> PISPIETVPVKLKPG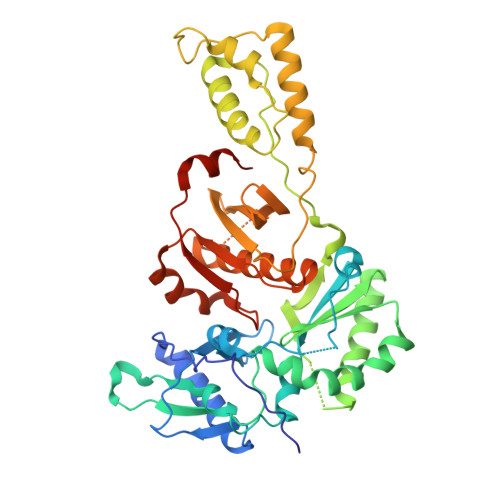MDGPKVKQWPLTEEKIKALVEICTEMEKEGKISKIGPENPYNTPVFAIKKKDSTKWRKLVDFRELNKRTQDFWEVQLGIPHPAGLKKKKSATVLDVGDAYFSVPLDEDFRKYTAFTIPSINNETPGIRYQYNVLPQGWKGSPAIFQSSMTKILEPFRKQNPDIVIYQYMDDLYVGSDLEIGQHRTKIEELRQHLLRWGLTTPDKKHQKEPPFLWMGYELHPDKWTVQPIVLPEKDSWTVNDIQKLVGKLNWASQIYPGIKVRQLCKLLRGTKALTEVIPLTEEAELELAENREILKEPVHGVYYDPSKDLIAEIQKQGQGQWTYQIYQEPFKNLKTGKYARMRGAHTNDVKQLTEAVQKITTESIVIWGKTPKFKLPIQKETWETWWTEYWQATWIPEWEFVNTPPLVKLWYQLEKEPIVGAETF>[2x]TRDQNGTWEMESNENFEGWMKALDIDFALRKIWVRLTQTLVIDQDGDNFKVKCTSTFWNYDVDFTVGVEFDEYTKSLDNRHVKALVTWEGDVLVCVQ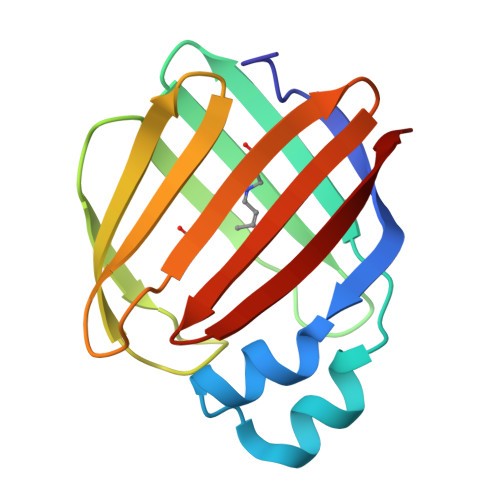KGEKENRGWKKWIEGDKLYLELTCGDQVCRQVFKKK> APTSSSTKKTQLQLEHLLLDLQMILNGINNYKNPKLTRMLTFCFYMPK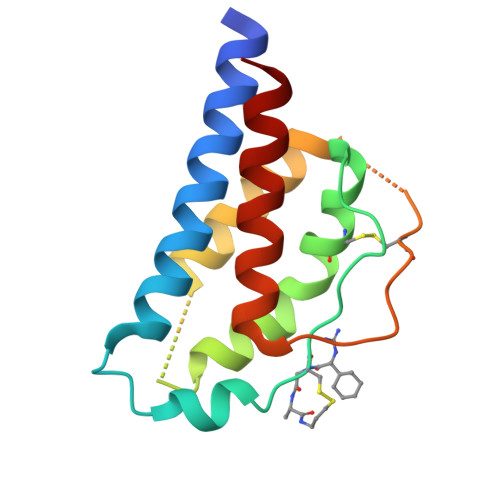KATELKHLQCLEEELKPLEEVLNLAQSKNFHLRPRDLISNINVIVLELKGSETTFMCEYADETATIVEFLNRWITFCQSIISTLT> MSATKSIVGEALEYVNIGLSHFLALPLAQRISLIIIIPFIYNIVWQLLYSLRKDRPPLVFYWIPWVGSAVVYGMKPYEFFEECQKKYGDIFSFVLLGRVMTVYLGPKGHEFVFNAKLADVSAEAAYAHLTTPVFGKGVIFDCPNSRLMEQKKFVKGALTKEAFKSYVPLIAEEVYKYFRDSKNFRLNERTTGTIDVMVTQPEMTIFTASRSLLGKEMRAKLDTDFAYLYSDLDKGFTPINFVFPNLPLEHYRKRDHAQKAISGTYMSLIKERRKNNDIQDRDLIDSLMKNSTYKDGVKMTDQEIANLLIGVLMGGQHTSAATSAWILLH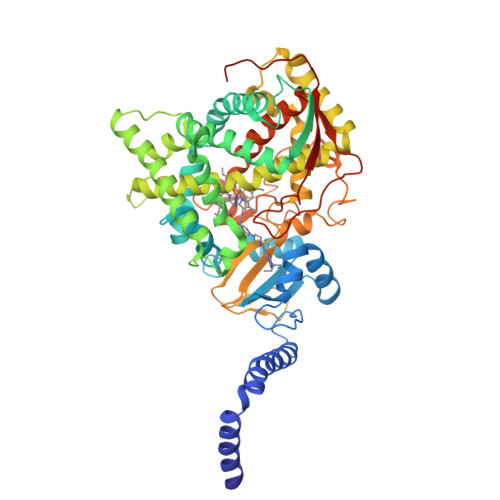LAERPDVQQELYEEQMRVLDGGKKELTYDLLQEMPLLNQTIKETLRMHHPLHSLFRKVMKDMHVPNTSYVIPAGYHVLVSPGYTHLRDEYFPNAHQFNIHRWNNDSASSYSVGEEVDYGFGAISKGVSSPYLPFGGGRHRCIGEHFAYCQLGVLMSIFIRTLKWHYPEGKTVPPPDFTSMVTLPTGPAKIIWEKRNPEQKIGGRHHHHHH> GHMATVKKLYFVPAGRCMLDHSSVNSALTPGKLLNLPVWCYLLETEEGPILVDTGMPESA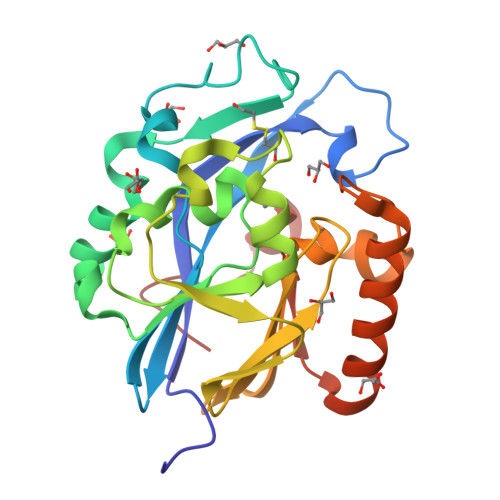VNNEGLFNGTFVEGQILPKMTEEDRIVNILKRVGYEPDDLLYIISSHLHFDHAGGNGAFTNTPIIVQRTEYEAALHREEYMKECILPHLNYKIIEGDYEVVPGVQLLYTPGHSPGHQSLFIETEQSGSVLLTIDASYTKENFEDEVPFAGFDPELALSSIKRLKEVVKKEKPIIFFGHDIEQEKSCRVFPEYI>[4x]SALEVYTPKEIFVANGTQGKLTCKF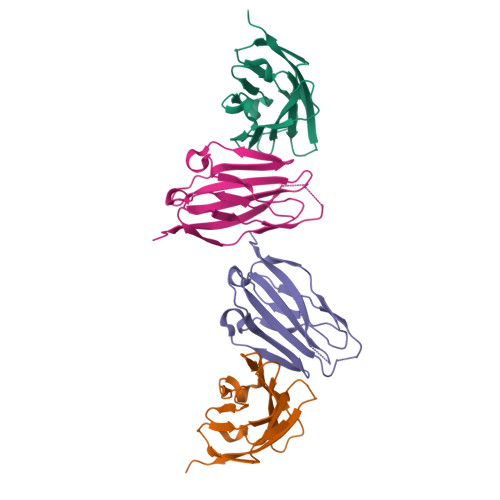KSTSTTGGLTSVSWSFQPEGADTTVSFFHYSQGQVYLGNYPPFKDRISWAGDLDKKDASINIENMQFIHNGTYICDVKNPPDIVGKTSHIRLYVVEKENLPVLEHHHHHH McrBC is an antiphage defense system of Escherichia coli that specifically cleaves invading DNA that are methylated. Furthermore, upon binding of the endonuclease McrC, a higher oligomeric form—tetradecamers of 12 McrB and 2 McrC protomers—is formed. GTP hydrolysis by McrBC bound to a recognition sequence powers DNA translocation, and convergence of two such complexes on the DNA results in nucleolytic cleavage. Here we present the structure of the AAA+ domain of McrB in complex with McrC at 3.6 Å resolution using cryo-electron microscopy (cryo-EM), which reveals the coupling between the endonuclease and the motor and the mechanism of activation of the GTPase.

The complex was formed in the presence of the GTP analog 5’-guanylyl imidodiphosphate (GNP). McrBΔNC is dumbbell shaped with the two hexameric McrBΔN rings tilted with respect to each other and sandwiching an McrC dimer. Three-dimensional (3D) classification resulted in nine major classes with varying tilt angle, indicative of conformational plasticity. The two protomers of McrC in the McrBΔNC complex are related to each other by a two-fold symmetry. The dimeric interface mainly constitutes helix H9 and has a total buried surface area of ~3000 Å2. The catalytic residues, Asp244, Asp257, and Lys259, are located close to the dimeric interface and aligned along the FA interface of McrB. A particularly interesting feature of McrBΔNC is that the McrC stalk blocks the pore of the McrB ring.

>[12x]MSKTESYCLEDALNDLFIPETTIETILKRLTIKKNIILQGPPGVGKTFVARRLAYLLTGEKAPQRVNMVQFHQSYSYEDFIQGYRPNGVGFRRKDGIFYNFCQQAKEQPEKKYIFIIDEINRANLSKVFGEVMMLMEHDKRGENWSVPLTYSENDEERFYVPENVYIIGLMNTADRSLAVVDYALRRRFSFIDIEPGFDTPQFRNFLLNKKAEPSFVESLCQKMNELNQEISKEATILGKGFRIGHSYFCCGLEDGTSPDTQWLNEIVMTDIAPLLEEYFFDDPYKQQKWTNKLLGDSSGSHHHHHH;>[2x]MEQPVIPVRNIYYMLTYAWGYLQEIKQANLEAIPGNNLLDILGYVLNKGVLQLSRRGLELDYNPNTEIIPGIKGRIEFAKTIRGFHLNHGKTVSTFDMLNEDTLANRIIKSTLAILIKHEKLNSTIRDEARSLYRKLPGISTLHLTPQHFSYLNGGKNTRYYKFVISVCKFIVNNSIPGQNKGHYRFYDFERNEKEMSLLYQKFLYEFCRRELTSANTTRSYLKWDASSISDQSLNLLPRMETDITIRSSEKILIVDAKYYKSIFSRRMGTEKFHSQNLYQLMNYLWSLKPENGENIGGLLIYPHVDTAVKHRYKINGFDIGLCTVNLGQEWPCIHQELLDIFDEYLK>YKWHYSGLNRWHGAGSTADFQKIIQERCDTYTQTIRPGSRSRNCQAIRQAFMSAFISKDPCKATKEDYNSLINLAPPTVPCGQQVFWSKTKELAHEYAKRRRLMTLEDTLLGYLADGLRWCGEPGSSDLNIWSCPDWRKDCRTNYLSVFWEVLSERFAESACNTVRVVLNGSLENAFDSMSIFGRVQAPNLRPQVELEAWLVHDTGKPP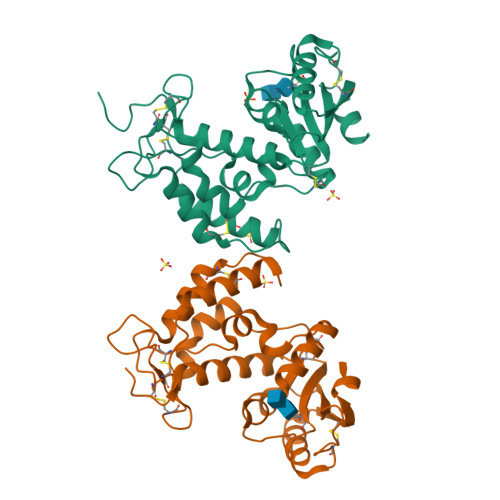SDSCSGSSIRKLKSILDGRNVKFRCMDNLSRDQFLQRS[2x]> QRLPLSKLVLTGERHYTRNDDIRQSILALGEPGTFMTQDVNIIQTQIEQRLPWIKQVSVRKQWPDELKIHLVEYVPIARWNDQHMVDAEGNTFSVPPERTSKQVLPMLYGPEGSANEVLQGYREMGQMLAKDRFTLKEAAMTARRSWQLTLNNDIKLNLGRGDTMKRLARFVEL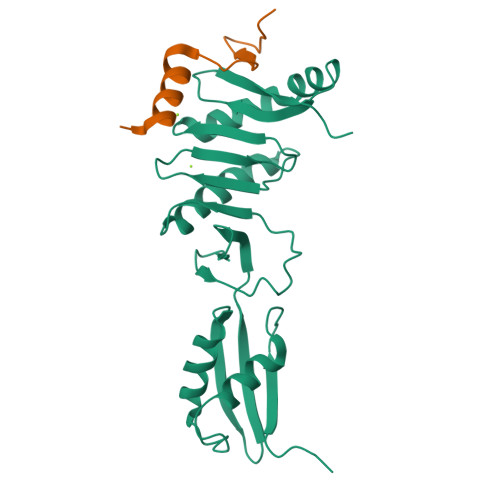YPVLQQQAQTDGKRISYVDLRYDSGAAVGWAPLPP;> NGGQEALEERARNELSMTRPGETFYRLVPDASKRA> MHRRGVGAGAIAKKKLAEAKYKERGTVLAEDQLAQMSKQLDMFKTNLEEFASKHKQEIRKNPEFRVQFQDMCATIGVDPLASGKGFWSEMLGVGDFYYELGVQIIEVCLALKHRNGGLITLEELHQQVLKGRGKFAQDVSQDDLIRAIKKLKALGTGFGIIPVGGTYLIQSVPAELNMDHTVVLQLAEKNGYVTVSEIKASLKWETERARQVLEHLLKEGLAWLDLQAPGEAHYWLPALFTDLYSQEITAEEAREALP;> GRIRAVGIVGIERKLEEKRKETDKNISEAFEDLSKLMIKAKEMVELSKSIANKIKDKQGDITEDETIRFKSYLLSMGIANPVTRETYGSGTQYHMQLAKQLAGILQVPLEERGGIMSLTEVYCLVNRARGMELLSPEDLVNACKMLEALKLPLRLRVFDSGVMVIELQSHKEEEMVASALETVSEKGSLTSEEFAKLVGMSVLLAKERLLLAEKMGHLCRDDSVEGLRFYPNLFMTQS;>MAMSFEWPWQYRFPPFFTLQPNVDTRQKQLAAWCSLVLSFCRLHKQSSMTVMEAQ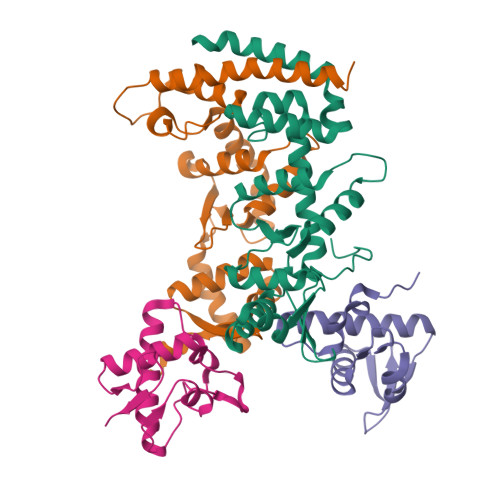ESPLFNNVKLQRKLPVESIQIVLEELRKKGNLEWLDKSKSSFLIMWR[2x]>MPKMIMVNKKASESQVMELEKRNYNNPVVLCGFAGSTPTGVLAASYIVETLGMHQVAHLISQHIPPVAVFVGGKLRHPFRIYANNSNTVLVAMCEVPISSAHIYEISNTLMNWIDQVGASEIVIMEGSPANGIPEERPVFAVAEKPKLDKFKKAGIQPADSAIIAGMGGGILNECLVRKITGLSFITPTSVDIPDPGAVLSIIEAINKAYNLKIKTDLLEEQVKALDEQIKKIEEQYKELQEKQKEPQSMYG[5x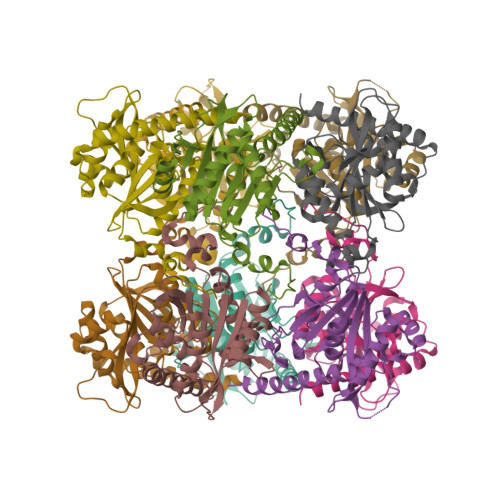]> RRELKLLLLGTGESGKSTFIKQMRIIHGS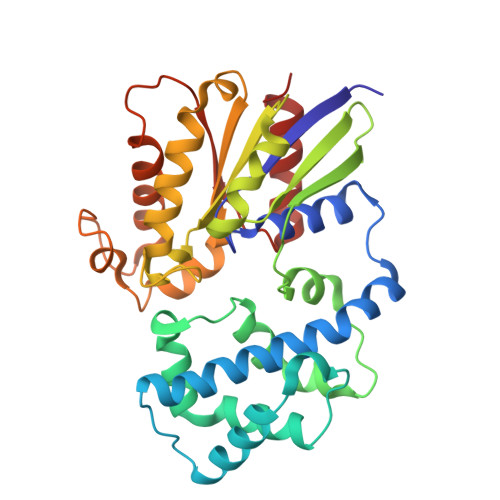GYSDEDKRGFTKLVYQNIFTAMQAMIRAMDTLKIPYKYEHNKAHAQLVREVDVEKVSAFENPYVDAIKSLWNDPGIQECYDRRREYQLSDSTKYYLNDLDRVADPSYLPTQQDVLRVRVPTTGIIEYPFDLQSVIFRMVDVGGQRSERRKWIHCFENVTSIMFLVALSEYDQVLVESDNENRMEESKALFRTIITYPWFQNSSVILFLNKKDLLEEKIMYSHLVDYFPEYDGPQRDAQAAREFILKMFVDLNPDSDKIIYSHFTCATDTENIRFVFAAVKDTILQ>GEVVDCHLSDMLQQLHSVNASKPSERGLVRQEEAEDPACIPIFWVSKWVDYSDKYGLGYQLCDNSVGVLFNDSTRLILYNDGDSLQYIERDGTESYLTVSSHPNSLMKKITLLKYFRNYMSEHLLKAGANITPREGDELARLPYLRTWFRTRSAIILHLSNGSVQINFFQDHTKLILCPLMAAVTYIDEKRDFRTYRLSLLEE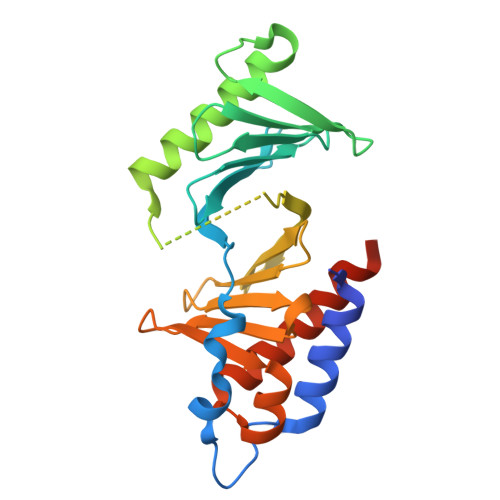YGCCKELASRLRYARTMVDKLLSSRSASNRLKAS[2x]>HHHHHHLVHVASVEKGRSYEDFQKVYNAIALKLREDDEYDNYIGYGPVLVRLAWHTSGTWDKHDNTGGSYGGTYRFKKEFNDPSNAGLQNGFKFLEPIHKEFPWISSGDLFSLGGVTAVQE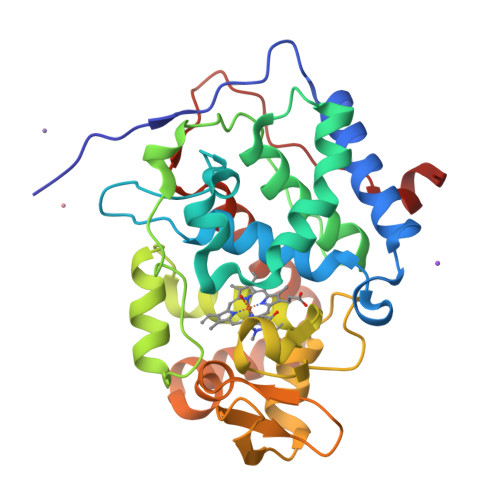MQGPKIPWRCGRVDTPEDTTPDNGRLPDADKDADYVRTFFQRLNMNDREVVALMGAHALGKTHLKNSGYEGPWGAANNVFTNEFYLNLLNEDWKLEKNDANNEQWDSKSGYMMLPTDYSLIQDPKYLSIVKEYANDQDKFFKDFSKAFEKLLENGITFPKDAPSPFIFKTLEEQGL[3x]> RCPEQELRLQRLERLPELARVLRNVFVSERKPALTMEVVCARMVDSCQTALSPGEMEKHLVLLAELLPDWLSLHRIRTDTYVK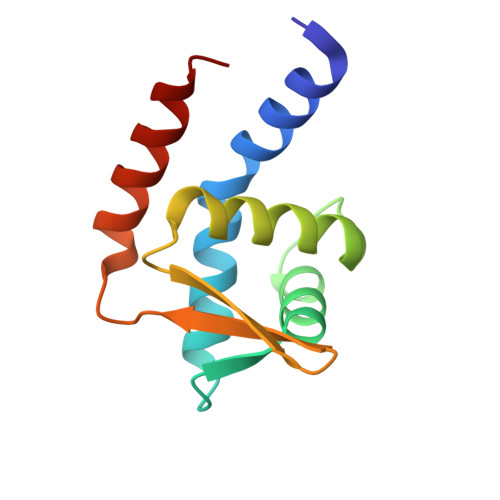LDKAVDLAGLTARLAHHVHAEGL>GSMALFSAQSPYINPIIPFTGPIQGGLQEGLQVTLQGTTKSFAQRFVVNFQNSFNGNDIAFHFNPRFEEGGYVVCNTKQNGQWGPEERKMQMPFQKGMPFELCFLVQRSEFKVMVNKKFFVQYQHRVPYHL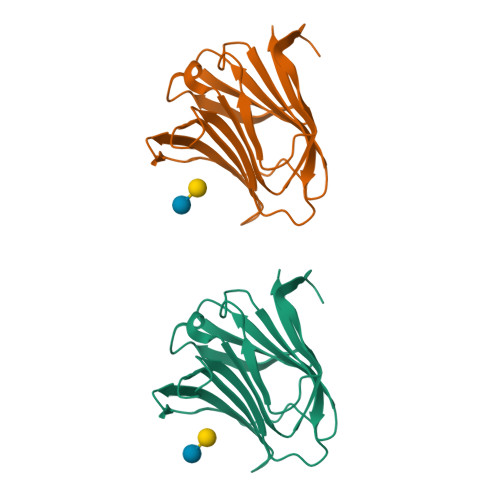VDTIAVSGCLKLSFITFQTQNFRPAHQA[2x]>[4x]MNRQQFIDYAQ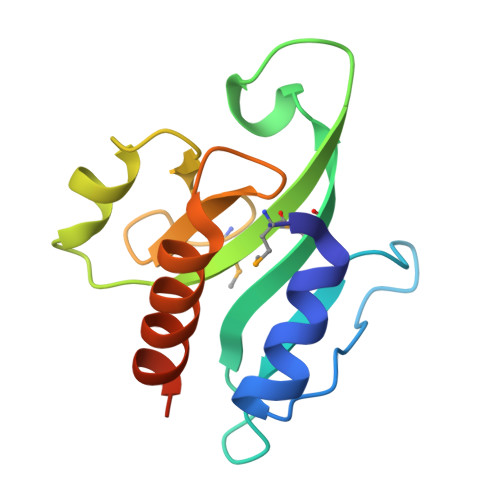KKYDTKPDHPWEKFPDYAVFRHSDNDKWYALLMDIPAEKIGINGDKRVDVIDLKVQPELVGSLRKKPGIYPAYHMNKEHWITVLLNGPLGAKEIHSLIEDSFQLTRLEHHHHHH To provide a molecular basis for designing better drugs targeting polymerases, African swine fever virus DNA Polymerase X (Pol X) was used as a model for the study. As the simplest DNA polymerase identified to date, Pol X belongs to the polymerase X family and is constituted of 174 amino acids. In this chemical reaction, metal-ion A (MeA) is a catalytic ion and decreases the pKa of 3′-OH, facilitating its attack on the α-phosphate of the incoming dNTP, and metal-ion B (MeB) stabilizes the dNTP-DNA-polymerase complex and increases the electrophilicity of the phosphorus center. To clearly understand the phosphodiester-bond-formation mechanism and the metal-ion catalysis of polymerases, we designed modified dNTP substrates with a chiral α-phosphorus center (α-P center) using a single selenium atom, without affecting the overall and local structures, to explore the absolute configuration inversion and probe the mechanisms of the metal ion–oxygen interactions.

In contrast, when using DNA-II (with 3′-OH) and dNTP (dGTP, dGTPαSe-I, or dGTPαSe-II), the DNA extension reaction took place to form DNApost, and the phosphodiester bond was formed (the after-reaction state, with the bond formation), followed by solving the absolute configuration of the Se-atom-modified P-center on DNApost in the product complex (the product-template–polymerase complex: nat-dG_pro, dGSe-I_pro, or dGSe-II_pro). In detail, we designed the crystallization trials with dGTP and dGTPαSe to form the products (DNApost: 5′-CGGATCC-dG-3′ and 5′-CGGATCC-dG(Se)-3′) from a self-complementary primer (5′-CGGATCC-3′) with one overhang 5′-dC-nucleotide. The 3′-OH attacked the incoming dGTP or dGTPαSe diastereomers in the crystallization conditions, thereby generating DNApost and forming the native and Se-modified product complexes. In the determined structures, the clear 2Fo-Fc electron-density maps and polder maps indicated that the three dNTPs were individually incorporated into the three DNApost products. The determined overall structures reached the atomic resolution, and the P-center configurations of these three product complexes (nat-dG_pro, dGSe-I_pro, and dGSe-II_pro) were solved as well. Though one nat-dG_pro complex and two dGSe_pro complexes belonged to P212121 and P21 space groups, respectively, their structures with the polymerase were virtually identical, especially the two dGSe_pro structures (RMSD: 0.2 Å). On the other hand, all three product-complex structures captured the reaction state at the post-polymerization level successfully.

>[2x]AGGMLTLIQGKKIVNHLRSRLAFEYNGQLIKILSKNIVAVGSLRREEKMLNDVDLLIIVPEKKLLKHVLPNIRIKGLSFSVKVCGERKCVLFIEWEKKTYQLDLFTALAEEKPYAIFHFTGPVSYLIRIRAALKKKNYKLNQYGLFKNQTLVPLKITTEKELIKELGFTYRIPKKRL> MAHHHHHHMTAFSDLLVVQEVSPRDGLQIEPTWVPTDKKIDLINQLSTMGFSRIEAGSFVSPKAIPNLRDGEEVFTGITRHKDIIYVGLIPNLKGALRAVEANANELNLVLSASQTHNLANMRMTKAQSFAGFTEIVEQLQGKTQFNGTVATTFGCPFEGKISEREVFSLVEHYLKLGIHN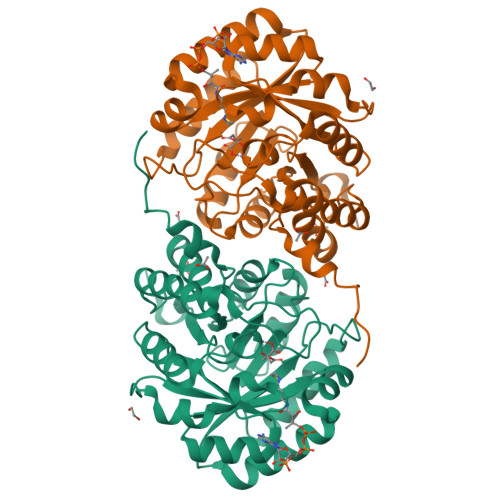ITLADTTGMANPVQVKRIVSHVLSLISPEQLTLHFHNTRGLGLTNVLAAYEVGARRFDAALGGLGGCPFAPGASGNICTEDLVNMCEEIGIPTTIDLDALIQLSRTLPALLGHDTPSQLAKAGRNTDLHPIPDYIKSLN> MASLEDGTYRLRAVTTHNPDPGVGGEYATVEGARQPVQAEPNTPPFFERQIWQVTRNADGQYTIKYQGLNAPFEYGFSYDQLEPNAPVIAGDPKEYILQLVPSTADVYIIRAPIQRVGVDVEVGVQGNTLVYKFFPVDGSGGDRPAWRFT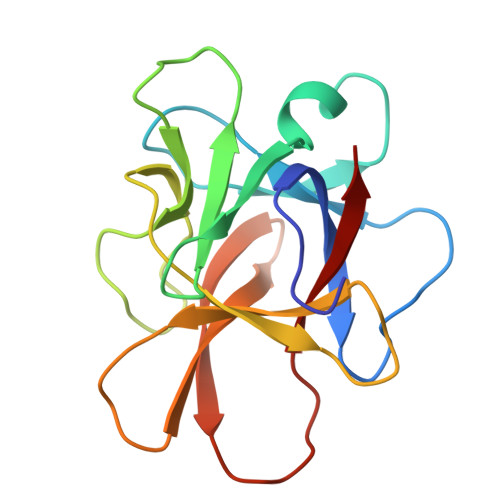RE> MADLSSRVNELHDLLNQYSYEYYVEDNPSVPDSEYDKLLHELIKIEEEHPEYKTVDSPTVRVGGEAQASFNKVNHDTPMLSLGNAFNEDDLRKFDQRIREQIGNVEYMCELKIDGLAVSLKYVDGYFVQGLTRGDGTTGEDITENLKTIHAIPLKMKEPLNVEVRGEAYMPRRSFLRLNEEKEKNDEQLFANPRNAAAGSLRQLDSKLTAKRKLSVFIYSVNDFTDFNA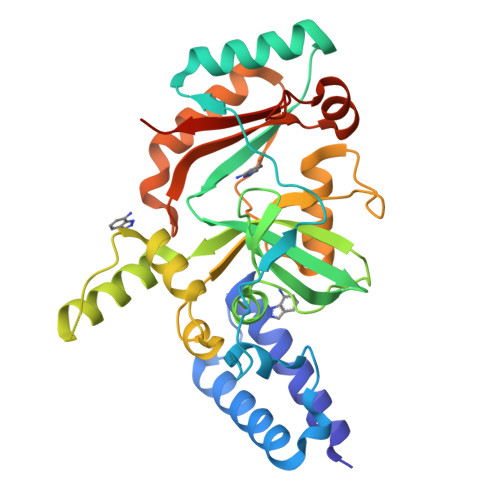RSQSEALDELDKLGFTTNKNRARVNNIDGVLEYIEKWTSQRESLPYDIDGIVIKVNDLDQQDEMGFTQKSPRWAIAYKFPAEEHHHHHH> DLYGESLDLRQRANVALHELKAYLQAAFQAVDRAIAQKSSNEMAIFLSETEATLAAPTQTKLQSALKKTIELNCFMTVPLDDLIYLLRLCDSALRQTESLDFSVQTSWGAQDVEQWLELLPNLEAAIRAARTSMRIMCGGREEKQLYSENAIEQALSLCKRLIDGIIMPLAELRNTSDTEELFKALSSCKRRILPLMTDAQKLLSMMSELIAKVDTSETVTNALEFAASQLLFIETANAERDSVIETQKFDGFRLVAMDMICQIFLLNPSQRQGIIDEILTSLEKLPLGKRARTFKLADGSSIQPVSALIMRLVQTSAGKDEGRGSSGRLDMTEGVQKVTGAKAFIIQSEAQGASQHSTAIRDLDTISTPLLETARNNASYVIKFIVNRALNSTKSGDTPYRNLLDLFVEDFITCLDNPDWPAAELLLRLLMLMMVGLVENDKSSIMAKNMALELLGTMCAAISKLRGHVRKMASALEADELSLFLSDLAASALELKSRPEHMVAWTGPYRATLEYLQSRSRFNEDAQLSSAMTFIISEWGSKICTCYDGYQDDVLERDQELGRLAYRLREMILDRKWLSTEYTYKDVSPLQAKLSYSIILLRSQFCEAFGAILNILLNSMASDQPTVRSKSLKSINQVMEADPTILDGDSVVVQLILRSSSDSSTQVRDSALGLISKCISLRPALEEKMTETVVNRFSDAGPGVRKRAMKLAKDIYLRNSNRVLRSAIANGLLHRVQDPEESVRDLARQVIEEIWFAPFHSGETSAASQISLSEHVILMVQTVKRGNVANVLDKVLQALLSPSSKTSQASMEVCRKLVGSMFDLIDNIDSNDASAPSGRDVLQVLMIFAKAEASLFTFEQLRLLRPYIASIGTSEDLTVSRAVVVIYRRVLPQLSSAHAQFLTDVRKELLPVVAKVPRALLDDVMACLWIISTLLGTYEPLA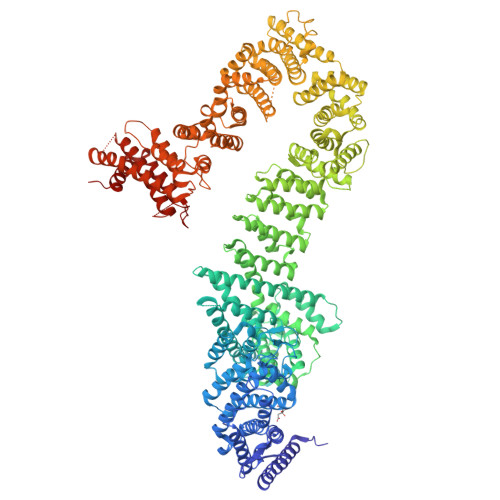RLVISSLKGIQKTRASAQVQPLDQLKIRQFDRYSLIVGMAGKHCNLDSHHEMFKEHFPKFSGASVSKLMVDIVVPFAAPSWPLDVRKPALDCVGLVCQSSPRNYVAANVYTAFQQVFDDQIPILETMVLRSLKEFLFSEEKRSEQEPEGPAGKDGESKKKRELTVIGGTNYDDVASATTHRFLKDITRIATSTQDDHAFLAVEVLASINRQGLVHPKETGVTFITLATSTHPRISELAFLEHKALHTKHETVIEREYAKAIQSIFAYQRDIVKDPRGATTNPFTPKLHLFMEVLKISKAKNRVKFLEKLVSQIDFDIAKLDMSEELPPHVQYSRFIIENLAFFEYVTVGEIHSLVAAMERLVASTGASVAQVIESEVFHLRIDVLDAPSSQSPNPDGQLRAEAQTQGQVNPLLPDIEYSRLRQLTAASMILLAIWEVRTYLRRLYSLGTNRRENSAKPAKPQVKDLARPPVKVQGVTGDKVWEEINNIMGALSGGRERMVRACKDLVELMSID> 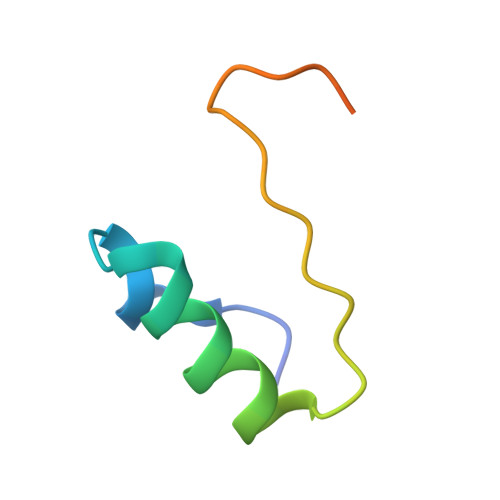MKTEWPELVGKSVEEAKKVILQDKPEAQIIVLPVGTIVTMGQQQQGM We describe here the use of an artificial cofactor employing the well‐known biotin‐streptavidin system to catalyze a Baylis‐Hillman reaction. As protein host, we chose streptavidin, as it can be easily crystallized and thereby supports the design process. There are several examples using streptavidin as the host for these cofactors, since its natural ligand biotin binds strongly (K d∼10−15 M) and is easy to modify with catalysts at the carboxylic acid group. No enzyme is known to naturally catalyze the Baylis‐Hillman reaction, a very versatile and atom‐economic C−C bond forming reaction for the production of various functionalized compounds and intermediates of active pharmaceutical ingredients (APIs).

We chose a derivative of DMAP as the artificial cofactor due to its low steric demand, which will facilitate its inclusion into the protein scaffold. The protein host around the cofactor was rationally designed on the basis of high‐resolution crystal structures obtained after each variation of the amino acid sequence. The location of the catalyst is in a shallow cavity at the surface of the protein. The system was evolved through repeated cycles of mutagenesis, activity tests, and structure determination. According to the presented structures and calculations the catalytically active site is too shallow to undergo interactions with 1.

>MASMTGGQQMGRDEAGITGTWYNQLGSTFIVTAGADGALTGTYESAAGKAESRYVLTGRYDSAPATDGSGTALGWTVAWKNNYRNAHSATTWSGQYVGGAEARINTQWLLTIGATEANGWASTYVGHDTFTKVKPSAASIDAAKKAGVNNGNPLDAVQQ[2x]3-[7-(2-hydroxyethyl)-9-(oxan-4-yl)-8-oxidanylidene-purin-2-yl]imidazo[1,2-a]pyridine-6-carbonitrile 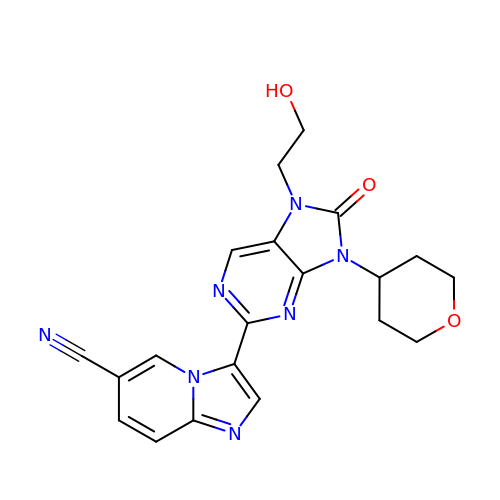| C20 H19 N7 O3 | RJIVCYWQVNETLQ-UHFFFAOYSA-N> SGDYRVQNTSLEAIVQNASSDNQGIQLSAVQAARKLLSSDRNPPIDDLIKSGILPILVHCLERDDNPSLQFEAAWALTNIASGTSEQTQAVVQSNAVPLFLRLLHSPHQNVCEQAVWALGNIIGDGPQCRDYVISLGVVKPLLSFISPSIPITFLRNVTWVMVNLCRHKDPPPPMETIQEILPALCVLIHHTDVNILVDTVWALSYLTDAGNEQIQMVIDSGIVPHLVPLLSHQEVKVQTAALRAVGNIVTGTDEQTQVVLNCDALSHFPALLTHPKEKINKEAVWFLSNITAGNQQQVQAVIDANLVPMIIHLLDKGDFGTQKEAAWAISNLTISGRKDQVAYLIQQNVIPPFCNLLTVKDAQVV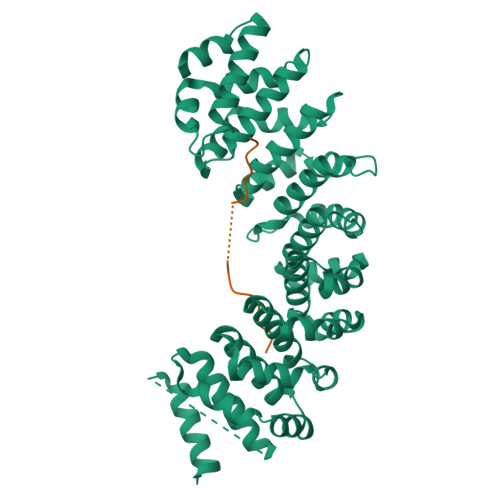QVVLDGLSNILKMAEDEAETIGNLIEECGGLEKIEQLQNHENEDIYKLAYEIIDQFFSSDDIDEDPSLVPEAIQGGTFGFNSSANVPTEGFQF;> RKARKRSHSPTKKLRYVKRRF>[4x]MLVVGSELQSDAQQLSAEAPRHGELQYLRQVEHILRCGFKKEDRTGTGTLSVFGMQARYSLRDEFPLLTTKRVFWKGVLEELLWFIKGSTNAKELSSKGVRIWDANGSRDFLDSLGFSARQEGDLGPVYGFQWRHFGAEYKDMDSDYSGQGVDQLQKVIDTIKTNPDDRRIIMCAWNPKDLPLMALPPCHALCQFYVVNGELSCQLYQRSGDMGLGVPFNIASYALL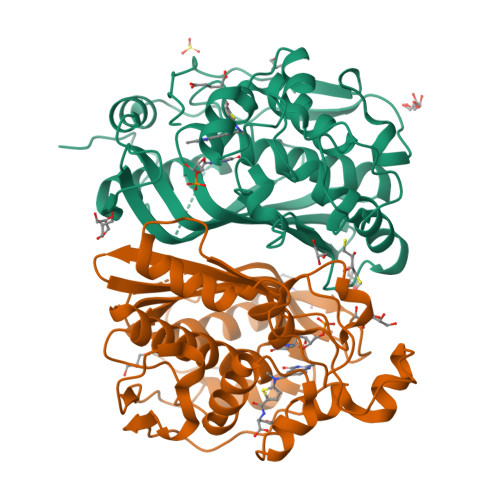TYMIAHITGLQPGDFVHTLGDAHIYLNHIEPLKIQLQREPRPFPKLKILRKVETIDDFKVEDFQIEGYNPHPTIKMEMAV Phage satellite P4 polarity suppression protein, Psu, a building block of the viral capsid, inhibits hexameric transcription termination factor, ρ, by presently unknown mechanisms. The ρ hexamer adopts an NTPase-inactive, washer-like, open-ring conformation until NTPs (preferentially ATP) are engaged and RNA is bound at the SBS, leading to ring closure and RNA entrapment inside the ring. Our cryogenic electron microscopy structures of ρ-Psu complexes show that Psu dimers clamp two inactive, open ρ rings and promote their expansion to higher-oligomeric states. ATPase, nucleotide binding and nucleic acid binding studies revealed that Psu hinders ρ ring closure and traps nucleotides in their binding pockets on ρ.

Complex IIexpanded is a complex II constellation, in which both ρ rings are augmented to the octamer level by incorporation of two additional peripheral ρ subunits, providing binding sites for two additional Psu dimers. A yet larger assembly, complex IIIexpanded, was observed in the ρ-ATPγS-Psu sample; the complex III arrangement leaves sufficient space in the center for incorporation of an additional subunit at each ρ ring (subunits 0 in Figs. 1e and 2b), and the rings are further expanded at the peripheries by two ρ subunits (subunits 7 and 8 in Figs. 1e and 2b); again, the additional ρ subunits generate binding sites for additional Psu dimers. Eight Psu dimers (purple and violet) bridge two open ρ nonamers, ρ(A) and ρ(B). The central Psu dimers of complex IIIexpanded are spaced close enough to reciprocally interact via their C-terminal α7 helices. In the largest ρ-ATPγS-Psu complex (complex IIIexpanded), additional contacts ensue between the dimerization region of the central Psu dimers and the NTDs of the central ρ subunits. We further refined complex II (ATP; global resolution 3.8 Å), complex IIexpanded (ATP; global resolution 3.6 Å), complex III (ATPγS; global resolution 3.65 Å), and complex IIIexpanded (ATPγS; global resolution 4.25 Å). The incorporation of additional ρ subunits supported by additional, bridging Psu dimers in complexes IIexpanded and IIIexpanded is facilitated by a further increase in the inter-subunit and ρ1-ρ6 rise values (10.5/11.1 Å and 52.4/55.5 Å, respectively); thus, the helical pitch in complexes IIexpanded and IIIexpanded is large enough to allow expansion by additional ρ protomers, as they can stack on preceding subunits in the stretched ρ rings. The most peripheral ρ subunits of the ρ(A)/ρ(B) rings in complexes IIexpanded and IIIexpanded are not stabilized by contacts to a Psu dimer, as no appropriately-spaced, unoccupied ρ subunit remains in the opposite ρ ring. While clearly defined in low-pass-filtered maps (6 Å resolution), density for these peripheral subunits is weak and fragmented in the cryoEM reconstructions refined to full resolution, suggesting that they are more flexibly connected or bound sub-stoichiometrically.

>[18x]MNLTELKNTPVSELITLGENMGLENLARMRKQDIIFAILKQHAKSGEDIFGDGVLEILQDGFGFLRSADSSYLAGPDDIYVSPSQIRRFNLRTGDTISGKIRPPKEGERYFALLKVNEVNFDKPENARNKILFENLTPLHANSRLRMERGNGSTEDLTARVLDLASPIGRGQRGLIVAPPKAGKTMLLQNIAQSIAYNHPDCVLMVLLIDERPEEVTEMQRLVKGEVVASTFDEPASRHVQVAEMVIEKAKRLVEHKKDVIILLDSITRLARAYNTVVPASGKVLTGGVDANALHRPKRFFGAARNVEEGGSLTIIATALIDTGSKMDEVIYEEFKGTGNMELHLSRKIAEKRVFPAIDYNRSGTRKEELLTTQEELQKMWILRKIIHPMGEIDAMEFLINKLAMTKTNDDFFEMMKRS;>[16x]MESTALQQAFDTCQNNKAAWLQRKNELAAAEQEYLRLLSGEGRNVSRLDELRNIIEVRKWQVNQAAGRYIRSHEAVQHISIRDRLNDFMQQHGTALAAALAPELMGYSELTAIARNCAIQRATDALREALLSWLAKGEKINYSAQDSDILTTIGFRPDVASVDDSREKFTPAQNMIFSRKSAQLASRQSV>[2x]GPHMEDENILRNAVNLQVLKFHYPEIESIIDIASHVAVYQFD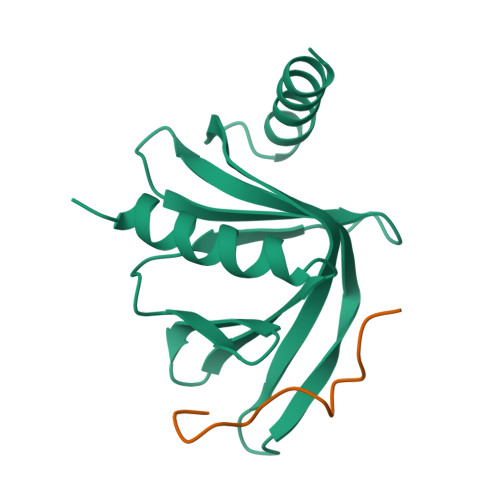VGSQKWLKTSIEGTFFLVKDQRARVGYVILNRNSPENLYLFINHPSNVHLVDRYLIHRTENQHVVGLWMFDPNDMSRIFNIVKESLLR;>SILYAGPTFTHSPAASNLPIPTFLHS[2x]> MAKFFIDRPIFAWVISIFIIAAGIFGIKSLPVSQYPSVAAPTITLHAIYPGASAQVMEGSVLSVIERNMNGVEGLDYMSTSADSSGSGSVSLTFTPDTDENLAQVEVQNKLSEVLSTLPATVQQYGVTVSKARSNFLMIVMLSSDVQSTEEMNDYAQRNVVPELQRIEGVGQVRLFGAQRAMRIWVDPKKLQNYNLSFADVGSALSAQNIQISAGSIGSLPAVRGQTVTATVTAQGQLGTAEEFGNVILRANTDGSNIYLKDVAKVGLGMEDYSSSTRLNGVN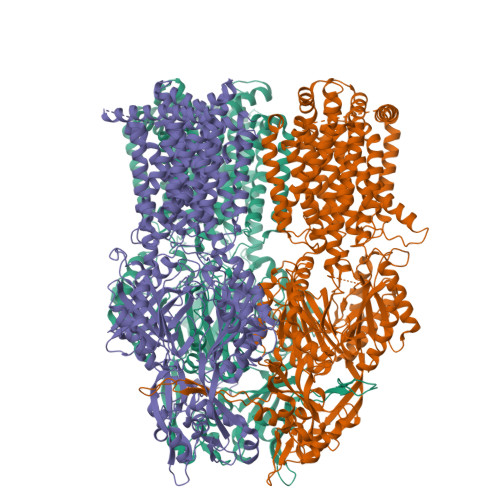TTGMAVMLSNSGNAMATAKAVKERLAVLEKYFPQGMSWKTPYDTSKFVEISIEKVIHTLIEAMVLVFVVMYLFLQNIRYTLIPTIVVPISLLGGFAFISYMGMSINVLTMFAMILVIGIVVDDAIVVVENVERIMAGEGLPPKEATKKAMGQISGAVIGITAVLISVFVPLAMFSGAAGNIYKQFALTMASSIAFSAFLALTLTPALCATMLKTIPKGHHEEKKGFFGWFNKKFDSWTHGYEGRVAKVLRKTFRMMVVYIGLAVVGVFLFMRLPTSFLPTEDQGFVMVSVQLPAGATKERTDATLAQVTQLAKSIPEIENIITVSGFSFSGSGQNMAMGFAIFKDWNERTASGSDAVAVAGKLTGMMMGTLKDGFGIAVVPPPILELGNGSGLSINLQDRNNTGHTALLAKRNELIQKMRASGLFDPSTVRAGGLEDSPQLKIDINRAAAAAQGISFADIRTALASALSSSYVSDFPNQGRLQRVMVQADEDARMQPADILNLTVPNKSGVAVPLSTIATVSWENGTEQSVRFNGYPSMKLSASPATGVSTGQAMEAVQKMVDELGGGYSFEWGGQSSEEAKGGSQTLILYGLAVAAVFLVLAALYESWSIPLAVILVIPLGLIGAAAGVTGRNLFEGLLGSVPSFANDIYFQVGFVTVMGLSAKNAILIIEFAKDLQAQGKSAVEAALEAARLRFRPIIMTSFAFILGVVPLYIAAGASSASQRAIGTTVFWGMLVGTLLSVFLVPLFYVVVRKFFKETAHEHEMAVRHASK>[2x]MGSSHHHHHHSQDPNSMPDNTIQWDKDADGIVTLTMDDPSGSTNVMNEAYIESMGKAVDRLVAEKDSITGVVVASAKKTFFAGGDVKTMIQARPEDAGDVFNTVETIKRQLRTLETLGKPVVAAINGAALGGGLEIALACHHRIAADVKGSQLGLPEVTLGLLPGGGGVTRTVRMFGIQNAFVSVLAQGTRFKPAKAKEIGLVDELVATVEELVPAAKAWIKEELKANPDGAGVQPWDKKGYKMPGGTPSSPGLAAILPSFPSNLRKQLKGAPMPAPRAILAAAVEGAQVDFDTASRIESRYFASLVTGQVAKNMMQAFFFDLQAINAGGSRPEGIGKTPIKRIGVLGAGMMGAGIAYVSAKAGYEVVLKDVSLEAAAKGKGYSEKLEAKALERGRTTQERSDALLARITPTADAADFKGVDFVIEAVFENQELKHKVFGEIEDIVEPNAILGSNTSTLPITGLATGVKRQEDFIGIHFFSPVDKMPLVEIIKGEKTSDEALARVFDYTLAIGKTPIVVNDSRGFFTSRVIGTFVNEALAMLGEGVEPASIEQAGSQAGYPAPPLQLSDELNLELMHKIAVATRKGVEDAGGTYQPHPAEA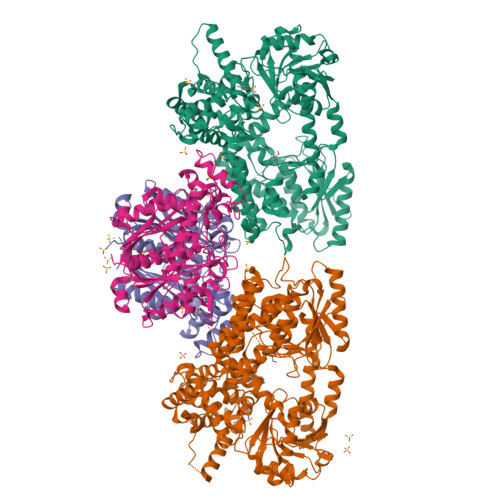VVEKMIELGRSGRLKGAGFYEYADGKRSGLWPGLRETFKSGSSQPPLQDMIDRMLFAEALETQKCLDEGVLTSTADANIGSIMGIGFPPWTGGSAQFIVGYSGPAGTGKAAFVARARELAAAYGDRFLPPESLLS;>[2x]MSEEAFIYEAIRTPRGKQKNGSLHEVKPLSLVVGLIDELRKRHPDLDENLISDVILGCVSPVGDQGGDIARAAVLASGMPVTSGGVQLNRFCASGLEAVNTAAQKVRSGWDDLVLAGGVESMSRVPMGSDGGAMGLDPATNYDVMFVPQSIGADLIATIEGFSREDVDAYALRSQQKAAEAWSGGYFAKSVVPVRDQNGLLILDHDEHMRPDTTKEGLAKLKPAFEGLAALGGFDDVALQKYHWVEKINHVHTGGNSSGIVDGAALVMIGSAAAGKLQGLTPRARIVATATSGADPVIMLTGPTPATRKVLDRAGLTVDDIDLFELNEAFASVVLKFQKDLNIPDEKLNVNGGAIAMGHPLGATGAMILGTMVDELERRNARRALITLCIGGGMGVATIIERV ethyl 2-[(2~{R})-1-[(4-methylphenyl)methyl]-3-oxidanylidene-piperazin-2-yl]ethanoate | C16 H22 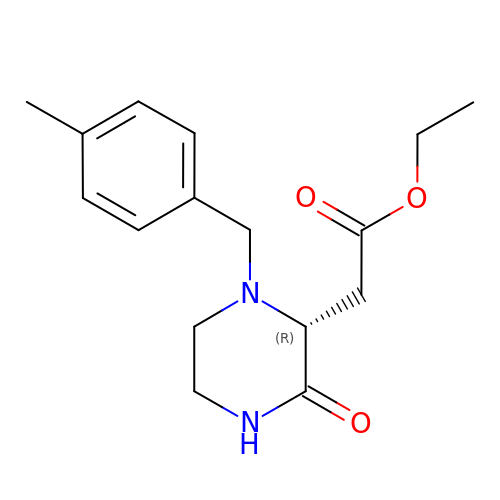N2 O3 | DPGLMZMGVNDMDP-CQSZACIVSA-N>[4x]MEEINTRLTFTVRRCAPELIVPAEPTPRELKPLSDIDDQEILRCHQKAIQFFRADPKMRHKNPASVIREALAKLLVFYYPFAGRIKESPVGKLMVDCTGEGVLFIEAEADVTLSQFGDPLQPPFPCIDELLYDVPGSSAILDAPIILYQVTRLSCGGFILAVRYNHAMTDAAGLLQFMSALGEIAGGATSPSIMPVWKRELLCSSDRPPIPITHDQIAAAKNETTQKSFFL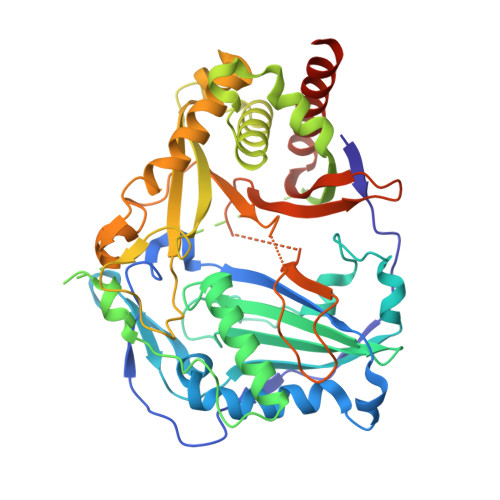TTTEISAFRRYVPTHLQSCTTFELLTACIWRCHTIALQPDPEEEMNMIWPVNVRNKFKFDPPLPAGYYGNLLAFSVAMSSARDLCSKPLGYALELVMKANHDVTKKKIGSVSDLLKPIKGPLPVRHDIVSDLIHGGHYSMEFGWGKATYTGPATGGIENNPGLTTYYVPYTNNKGESGVVVPLLLRSAVMTRFVNEINNMLAQVQNNEAIQEHKSPASSKL> GAMGSAVGDGPPRVDFPRSRLRFKEKLGEGQFGEVHLCEVDSPQDLVSLDFPLNVRKGHPLLVAVKILRPDATKNARNDFLKEVKIMSRLKDPNIIRLLGVCVQDDPLCMITDYMENGDLNQFLSAHQLEDKAAEGAPGDGQAAQGPTISYPMLLHVAAQIASGMRYLATLNFVHRDLATRNCLVGENFTIKIADFGMSRNLYAGDYYRVQGRAVLPIRWMAWECILMGKFTTASDVWAFGVTLWEVLMLCRAQPFGQLTDEQVIENAGEFFRDQGRQVYLSRPPACPQGLYELMLRCWS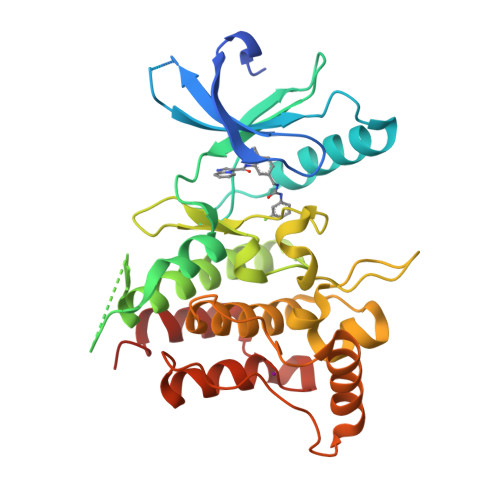RESEQRPPFSQLHRFLAEDALNTV>[2x]MRSRRVDVMDVMNRLILAMDLMNRDDALRVTGEVREYIDTVKIGYPLVLSEGMDIIAEFRKRFGCRIIADAKVADIPETNEKICRATFKAGADAIIVHGFPGAD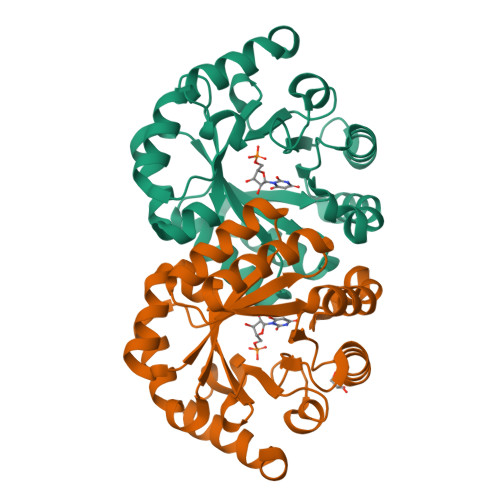SVRACLNVAEEMGREVFLLTEMSHPGAEMFIQGAADEIARMGVDLGVKNYVGPSTRPERLSRLREIIGQDSFLISPGVGAQGGDPGETLRFADAIIVGRSIYLADNPAAAAAGIIESIKDLLNP>GSMKIDVVTIFPEYLQPVRQSLPGKAIDAGLVDVAVHDLRRWTHDVHKSVDDSPYGGGPGMVMKPTVWGDALDEICTSETLLVVPTPAGYPFTQETAWQWSTEDHLVIACGRYEGIDQRVADDAATRMRVREVSIGDYVLNGGEAAALVIIEAVLRLVPGVLG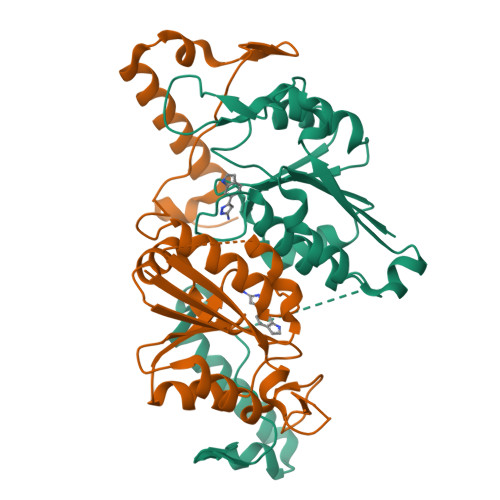NALSAQEDSHSEGMASLLEGPSYTRPPSWRGMDVPPVLLSGDHAKIAAWRAEQSRQRTIERRPDLLGFDSPTGEHGGDGLS[2x]> MGSVWFRNRYWWYRSLYDDYVAREAKLAFGIAAFIWLPHYYWGIHLNRAF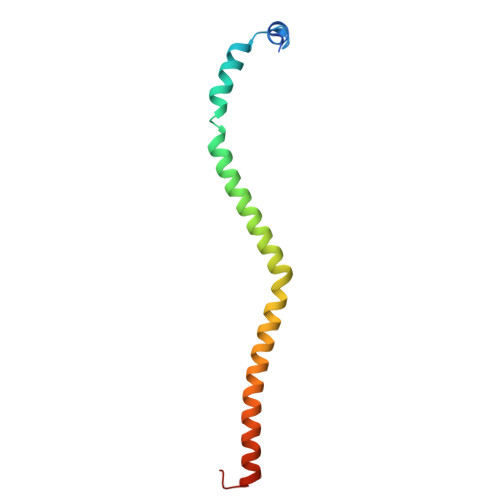EVNFSHRNYAHEWGPRRNRLAHSLEFEQFDMILENWQDLEDEYAQRGDGMLKK> MKLKKIVFTLIALGLFSCKTTSVLVKNEPQLKTPKNVILLISDGAGLSQISSTFYFKSGTPNYTQFKNIGLIKTSSSREDVTDSASGATAFSCGIKTYNAAIGVADDSTAVKSIVEIAALN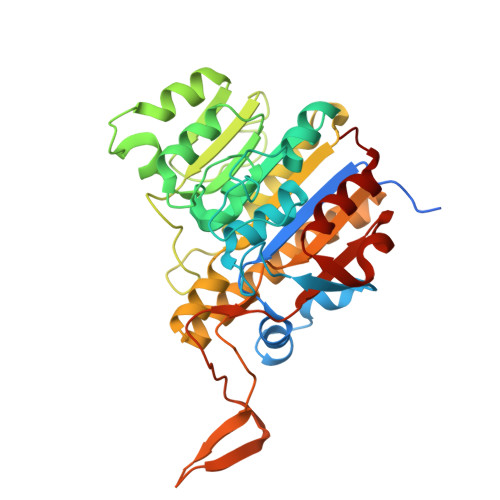SIKTGVVATSSITHATPASFYAHALNRGLEEEIAMDMTESDLDFFAGGGLNYFTSRSDSKDVLAILKGNQFTINTTGLTDFSSIASNRKMGFLLADEAMPTMEKGRGNFLSAATDLAIQFLSKDNSAFFIMSEGSQIDWGGHANNASYLISEINDFDDAIGTALAFAKSDGNTLVIVTSDHETGGFTLAAKSNKREDGSEYSDYTEIGPTFSTGGHSATLIPVFAYGPGSEEFIGIYENNEIFHKILKVTKWNQ>[2x]GSHMKPVIVKNVRIGEGNPKIVVPIVAPTAEDILAEATASQTLDCDLV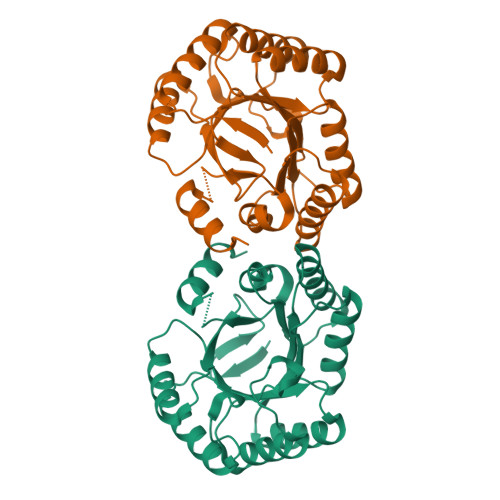EWRLDYYENVADFSDVCNLSQQVMERLGQKPLLLTFRTQKEGGEMAFSEENYFALYHELVKKGALDLLDIELFANPLAADTLIHEAKKAGIKIVLCNHDFQKTPSQEEIVARLRQMQMRQADICKIAVMPQDATDVLTLLSATNEMYTHYASVPIVTMSMGQLGMISRVTGQLFGSALTFGSAQQASAPGQLSVQVLRNYLKTFEQNK>MDTPRPQLLDFQFHQNNDSFTLHFQQRLILTHSKDNPCLWIGSGIADIDMFRGNFSIKDKLQEKIALTDAIVSQSPDGWLIHFSRGSDISATLNISADDQGRLLLELQNDNLNHNRIWLRLAAQPEDHIYGCGEQFSYFDLRGKPFPLWTSEQGVGRNKQTYVTWQADCKENAGGDYYWTFFPQPTFVSTQKYYCHVDNSCYMNFDFSAPEYHELALWEDKATLRFECADTYISLLEKLTALLGRQPELPDWIYDGVTLGIQGGTEVCQKKLDTMRNAGVKVNGIWAQDWSGIRMTSFGKRVMWNWKWNSENYPQLDSRIKQWNQEGVQFLAYINPYVASDKDLCEEAAQHGYLAKDASGGDYLVEFGEFYGGVVDLTNPEAYAWFKEVIKKNMIELGCGGWMADFGEYLPTDTYLHNGVSAEIMHNAWPALWAKCNYEALEETGKLGEILFFMRAGSTGSQKYSTMMWAGDQNVDWSLDDGLASVVPAALSLAMTGHGLHHSDIGGYTTLFEMKRSKELLLRWCDFSAFTPMMRTHEGNRPGDNWQFDGDAETIAHFARMTTVFTTLKPYLKEAVALNAKSGLPVMRPLFLHYEDDAHTYTLKYQYLLGRDILVAPVHEEGRSDWTLYLPEDNWVHAWTGEAFRGGEVTVNA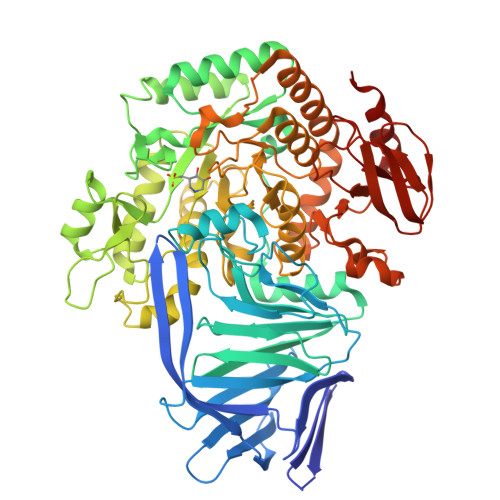PIGKPPVFYRADSEWAALFASLKSILEHHHHHH[2x]> MENDPNLFVALYDFVASGDNTLSITKGEKLRVLGYNHNGEWCEA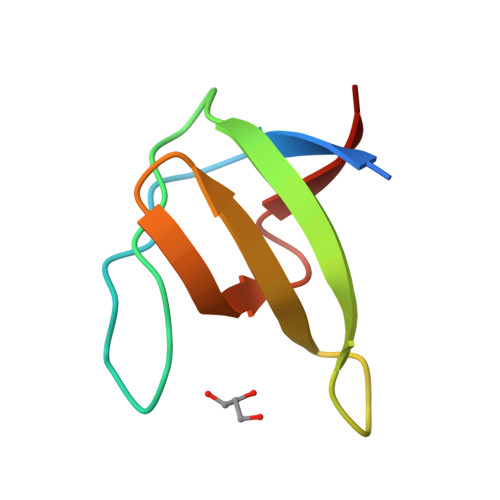QTKNGQGWVPSTYITPVNS> MRIIILALLIVCTIINYYCAVQNNGNKSLNVMPTCSMPGNDSDSNDNETGDVDNDKNNELGNANDNNEMNNENAESKNMQGENSNNQEQLNENVHANDDAMYEGTPSSDNPPQENVD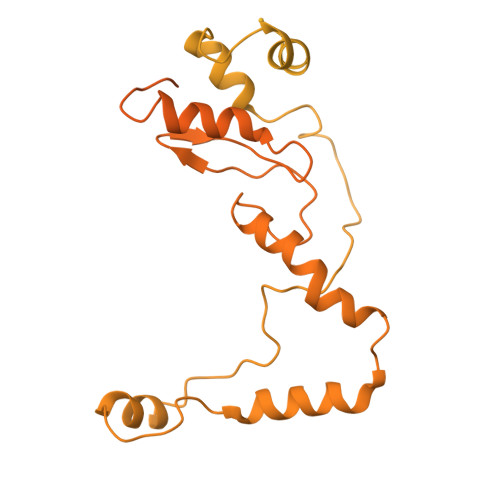ANNNEQEYGPPQEEPVSENNVENVEVATDDSGNDNINNNDNFNNNDNYNDNDNFNEEPPSDDGNKNEDELTEGNQSDDKPMNEEEATINEMGKITNPFEDMLKGKVDDMDIGKMMNKDNLQSFLSSLTGNKDGSGKNPLSDMMNIFGVPQTGKEGAEGGVNKENQMKQINELKDKLETMLKGAGVNVDKIKDSIKNNDLLKNKQLLKEAISKLTLDPSMMNMLNNKDGANGKPFDINPDSMMKMFNALSNENGNLDDLKMKPTDGSFDSFNDGVDNNLVPSNPKGQNNNEEDDEEGGDDDDYDDKSFVVNSKYADNSFEDKFNTFDEKDDDVKYELFGENEEAEELNNNTTTASSKGDANNSVNTQEGEGEEESFSANEENINNNNNHNNKNYNNYNTSQQEEDDNSFNENDEPLISSSQFDNNKKNKMSVSTHNKKSKNLMDSLDLESTNYGSNSSSSMSNNYNSKNKNSKKNNKKKSSQKDYIRTDGKVSFDMATLQKTIKNFGGADNEIVQNILKKYVTIDNDDDNDADEDEDEDDDDDDDLDEDEFSVKDIKKLIEEGILDYEDLTENELRKLAKPDDNFYELSPYASDEKDLSLNETSGLTNEQLKNFLGQNGTYHMSYDSKSIDYAKQKKSEKKEDQQEDDDGFYDAYKQIKNSYDGIPNNFNHEAPQLIGNNYVFTSIYDTKENLIKFLKKNSEYDLYDDDDKEGGNFKSPLYDKYGGKLQKFKRQRAFNILKQWRAKEKKLKEKKKKEEMEENKEFDFSKNYNFSSKNDGGVTMFSKDQLEDMVKNFGGKPSAHVTDSFSRKENPFVPTNTKNNSNDDDDMDNGYVTFDGKNKVSENDDDEKGNNNDDENDNDDSNDEEELDEEEDDN> MAEQVALSRTQVCGILREELFQGDAFHQSDTHIFIIMGASGDLAKKKIYPTIWWLFRDGLLPENTFIVGYARSRLTVADIRKQSEPFFKATPEEKLKLEDFFARNSYVAGQYDDAASYQRLNSHMNALHLGSQANRLFYLALPPTVYEAVTKNIHESCMSQIGWNRIIVEKPFGRDLQSSDRLSNHISSLFREDQIYRIDHYLGKEMVQNLMVLRFANRIFGPIWNRDNIACVILTFKEPFGTEGRGGYFDEFGIIRDVMQNHLLQMLCLVAMEKPASTNSDDVR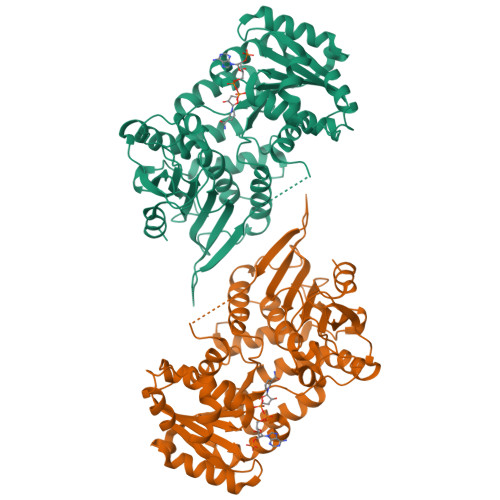DEKVKVLKCISEVQANNVVLGQYVGNPDGEGEATKGYLDDPTVPRGSTTATFAAVVLYVENERWDGVPFILRCGKALNERKAEVRLQFHDVAGDIFHQQCKRNELVIRVQPNEAVYTQMMTKKPGMFFNPEESELDLTYGNRYKNVKLPDAYERLILDVFCGSQMHFVRSDELREAWRIFTPLLHQIELEKPKPIPYIYGSRGPTEADELMKRVGFQYEGTYKWVNPHKL> MNTPEHMTAVVQRYVAALNAGDLDGIVALYASDATVTESFRPPFTGTEAIREFYANSLKLPLAV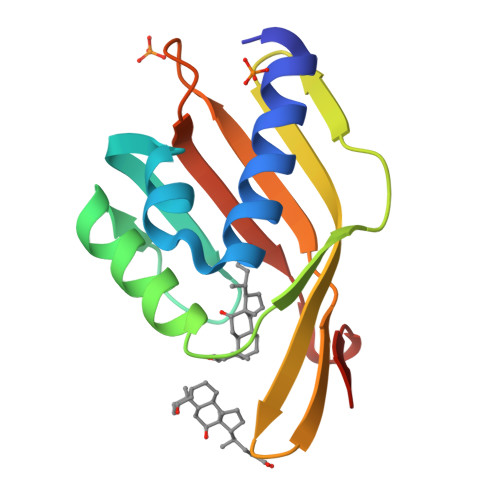ELTQEVRAANGEAAFAFIVSFEYQGRKTVVAPIDHFRFNGAGKIVYAQALFGEKNIHAGA>MKFSKEQFDYSLYLVTDSGMIPEGKTL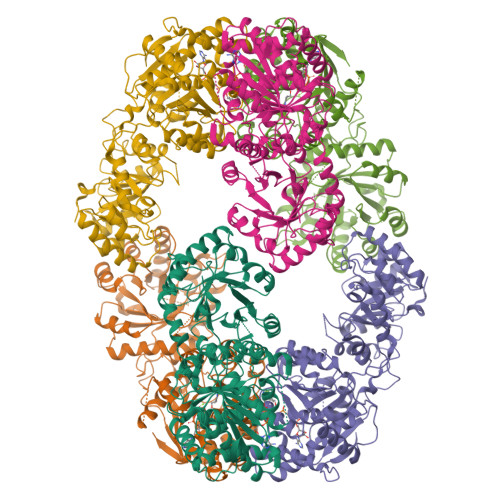YGQVEAGLQNGVTLVQIREKDADTKFFIEEALQIKELCHAHNVPLIINDRIDVAMAIGADGIHVGQDDMPIPMIRKLVGPDMVIGWSVGFPEEVDELSKMGPDMVDYIGVGTLFPTLTKKNPKKAPMGTAGAIRVLDALERNNAHWCRTVGIGGLHPDNIERVLYQCVSSNGKRSLDGICVVSDIIASLDAAKSTKILRGLIDKTDYKFVNIGLSTKNSLTTTDEIQSIISNTLKARPLVQHITNKVHQNFGANVTLALGSSPIMSEIQSEVNDLAAIPHATLLLNTGSVAPPEMLKAAIRAYNDVKRPIVFDPVGYSATETRLLLNNKLLTFGQFSCIKGNSSEILGLAELNKERMKGVDASSGISNELLIQATKIVAFKYKTVAVCTGEFDFIADGTIEGKYSLSKGTNGTSVEDIPCVAVEAGPIEIMGDITASGCSLGSTIACMIGGQPSEGNLFHAVVAGVMLYKAAGKIASEKCNGSGSFQVELIDALYRLTRENTPVTWAPKLTHT[3x]N-[2-(BENZHYDRYLOXY)ETHYL]-N,N-DIMETHYLAMINE 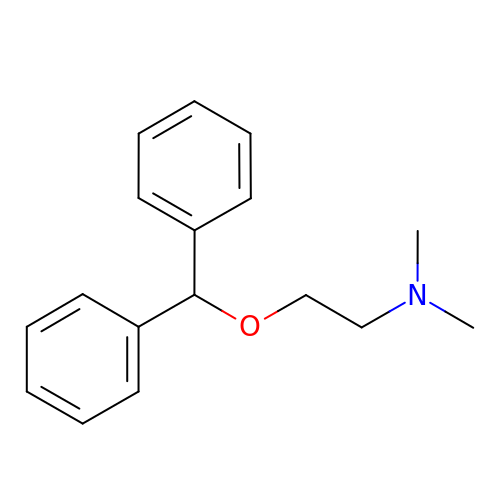| C17 H21 N O | ZZVUWRFHKOJYTH-UHFFFAOYSA-N> MLYEDPPDQKTSPSGKPATL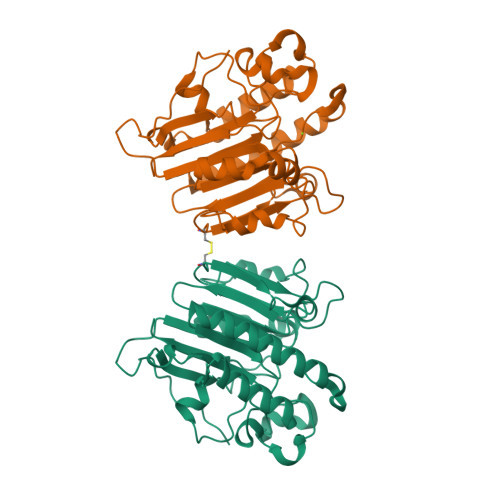KICSWNVDGLRAWIKKKGLDWVKEEAPDILCLQETKCSENKLPAELQELPGLSHQYWSAPSDKEGYSGVGLLSRQCPLKVSYGIGDEEHDQEGRVIVAEFDSFVLVTAYVPNAGRGLVRLEYRQRWDEAFRKFLKGLASRKPLVLCGDLNVAHEEIDLRNPKGNKKNAGFTPQERQGFGELLQAVPLADSFRHLYPNTPYAYTFWTYMMNARSKNVGWRLDYFLLSHSLLPALCDSKIRSKALGSDHCPITLYLAL>[4x]XDYLRELLKLELQAIKQYREA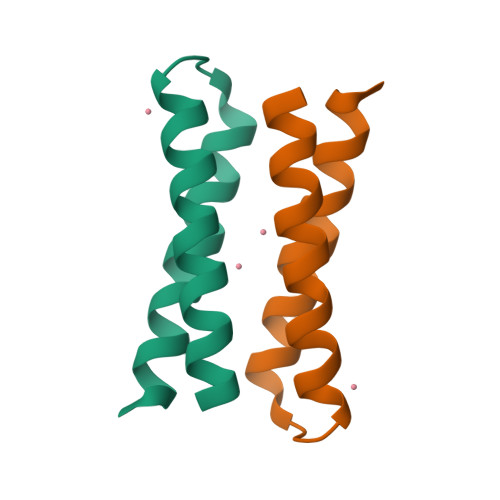LEYVKLPVLAKILEDEEKHIEWLETILGX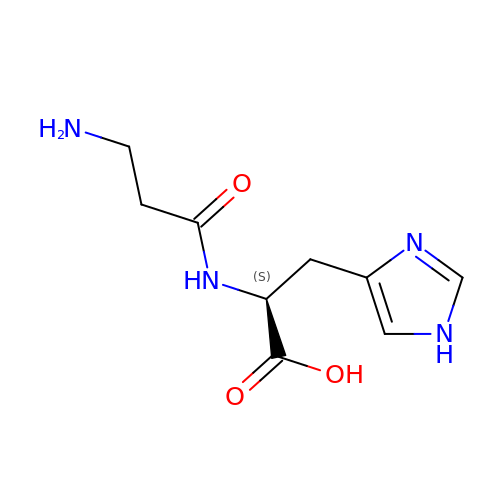(2~{S})-2-(3-azanylpropanoylamino)-3-(1~{H}-imidazol-4-yl)propanoic acid | C9 H14 N4 O3 | CQOVPNPJLQNMDC-ZETCQYMHSA-N>[6x]GSSPNLRYPIADVSGGIGMSPNYRFRQSMWIGIVSYSGSGLNWRVQVNSDIFIVDDYIHICLPAFDGFSIADGGDLSLNFVTGLLPPLLTGDTEPAFHNDVVTYGAQTVAIGLSSGGTPQYMSKNLWVEQWQDGVLRLRVEGGGSITHSNSKWPAMTVSYPRSFT;>GSSVTVHSSEPEVRIPENNPVKLSCAYSGFSSPRVEWKFDQGDTTRLVCYNNKITASYEDRVTFLPTGITFKSVTREDTGTYTCMVSEEGGNSYGEVKVKLIVL[6x]

Junctional adhesion molecule-A (JAM-A) is an IgSF member that mediates cell-cell contacts and serves as a receptor for mammalian orthoreovirus (reovirus) and feline calicivirus. At the virion fivefold symmetry axes, the trimeric attachment protein, σ1, extends from pentameric turrets formed by the λ2 protein. The σ1 molecule is about 480 Å in length and composed of a filamentous N-terminal tail and a globular C-terminal head. The σ1 head binds to JAM-A.

To define the structural basis of σ1-JAM-A interactions, we crystallized a complex of the head domain of T3D σ1 and the D1 domain of human JAM-A (hJAM-A) and determined its structure at 3.4 Å resolution. A T3D σ1 fragment comprising the head domain and one β-spiral of the tail (σ1H; residues 293–455) and the D1 domain of hJAM-A (D1; residues 28–129) were purified using glutathione S-transferase (GST)-affinity purification. The crystallographic asymmetric unit consists of two σ1H trimers, each bound to three D1 monomers. The crystallized complex consists of a σ1H trimer ligated by three D1 monomers. When viewed along the three-fold non-crystallographic symmetry axis, its overall structure resembles a three-bladed propeller, with σ1H forming the hub and D1 forming the blades. Each D1 monomer interacts with one σ1H monomer, making extensive contacts that shield a combined area (the sum of contact areas on both proteins) of 1622 Å2 from solvent. D1 residues involved in contact formation are located at the most membrane-distal (top) part of the domain and on the face that mediates homodimer formation. Reovirus σ1H engages JAM-A D1 using two main contact areas: a larger region centered at the D–E loop and its 310 helix, just below the β-barrel, and a smaller region formed by the top of the β-spiral and the α-helix. Contacts are largely polar, featuring numerous hydrogen bonds and two salt bridges. Instead, extensive hydrophobic interactions with substantial surface complementarity are found, indicating that this area also plays an important role in defining specificity and providing high affinity.> MVMDVVSRLHQKYGAEVEKALVRYLSIGLAEDFREAVLYQVK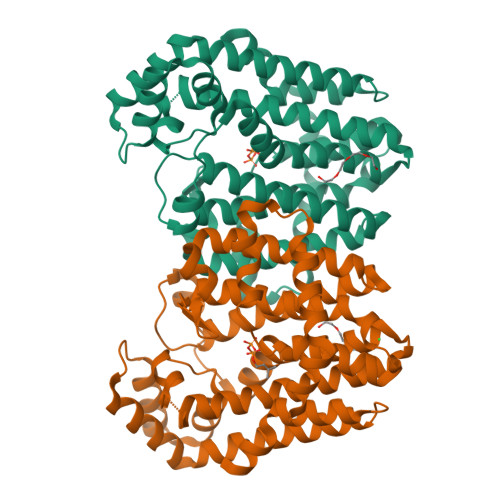TGGKRLRPLLTLAAAEAVSGQWRPALPAAAIVELIHNYSLIYDDIIDRGDVRRGLPTVRKAFGDNAAILVGIWYREAIEEAVLDTPKPTLFAKEVAEVIKAIDEGERLDILFEAAGRSDPYFVQARWREVTLDDYIKMVSLKTGALIAAAAKWGVLSVSDDRGLAEAAWNFGMAAGVAFQIIDDVLDIYGDPKKFGKEIGKDIKEHKRGNAVVAVALSHLGEGERRRLLEILAREVVEEADVREAVALLDSVGAREEALRLAARYREEAERHLAKIPNNGTLKELLDFIVAREYAENLYFQSHHHHHHWSHPQFEK> GPGSEFSEAISIDLLQKKGLVKAVNIAVDLIVAHFGTSRDPGVKAKLGNSSVSPNVGHLVLKYLCPAVRAVLEDGLKAFVLDVIIGQRKNMPWSV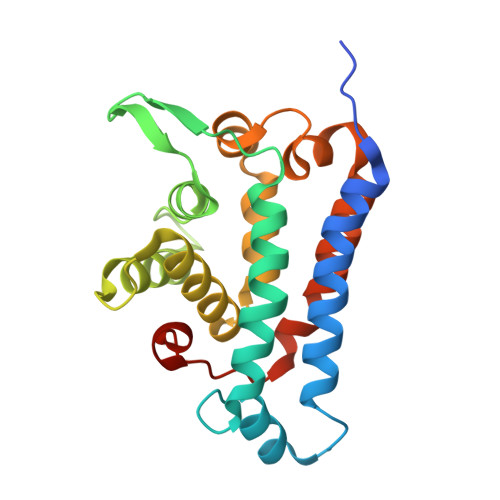VEASTQLGPSTKVLHGLYNKVSQFPELTSHTMRFNAFILGLLNIRSLEFWFNHLYNHEDIIQTHYQPWGFLSAAHTVCPGLFEELLLLLQPLALLPFSLDLLFQHRLLQS> STENEKSRSLPAERNPLYKDDTLDHT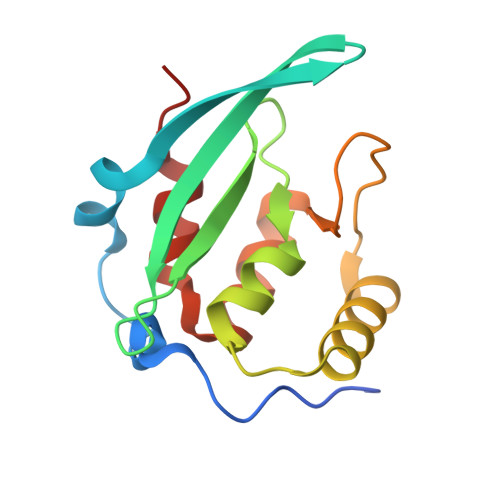PLIPKCRAQVIEFPDGPATFVRLKCTNPESKVPHFLMRMAKDSSISATSMFRSAFPKATQEEEDLEMRWIRDNLNPIEDKRVAGLWVPPADALALAKDYSMTPFINALLEASST>GGUGCUGGUGGUUGGCACUCCUGGUUUCCAGGACGGGGUUCAAAUCCCUGCGGCGUC[2x]

The AS and TSL stack to form one continuous helical stack containing four GU base pairs, while the AC and DSL form another. The two helices are held in a roughly perpendicular orientation by interactions between the elements that are analogous to the D and T loops in tRNA.

To crystallize human mascRNA, we strategically mutated adenine to guanine at the second position (A2G) and removed the UCCA sequence from the 3′ terminus. This approach was instrumental in achieving the desired crystalline structure. Compared to the tRNA structure, the TSL of mascRNA almost perfectly overlaps, whereas the DSL of mascRNA is shorter, with its lower half deviating by ~15°. Furthermore, the T loop of mascRNA exhibits a key interaction between nucleotides U39–A43 and two guanines in the D loop, echoing the tRNA’s elbow region. U39 and U40, the leading nucleotides of the T loop, are integrated into the stacking configuration of the T stem, and the nucleotide C41 pairs with G15 in the DSL through Watson–Crick base pairing. G14 is interposed between A42 and A43, creating a continuous stacking pattern that bridges the gap between these two nucleotides. In the L-shaped structure of tRNA, the elbow region is stabilized by interactions between the V loop and the D stem. However, mascRNA lacks many of these key stabilizing interactions. Instead, it has a distinctive triple base interaction that provides structural integrity. This interaction involves a hydrogen bond from the N4 of C16 to the N1 of A44, along with a base pair formed between G10 and C16.> GSHMAKEEIIWESLSVDVGSQGNPGIVEYKGVDTKTGEVLFEREPIPIGTNNMG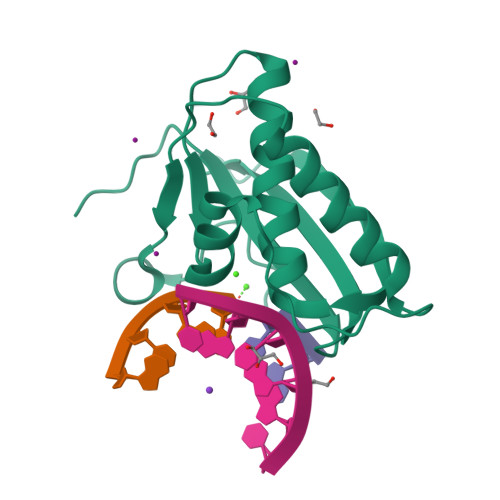EFLAIVHGLRYLKERNSRKPIYSDSQTAIKWVKDKKAKSTLVRNEETALIWKLVDEAEEWLNTHTYETPILKWQTDKWGEIKADYGRK>GSDGDYDYLIKFLALGDSGVGKTSVLYQYTDGKFNSKFITTVGIDFREKTIYRNDKRIKLQLWDTAGLERFRSLTTAFFRDAMGFLLLFDLTNEESFLNVRNWISQLKTHAYSENPDIVLCGNKSDLEDERVVAAAEARQLAEHYGIPYFETSAANGTNISQAIEMLLDLIMKRMERSVDKS[16x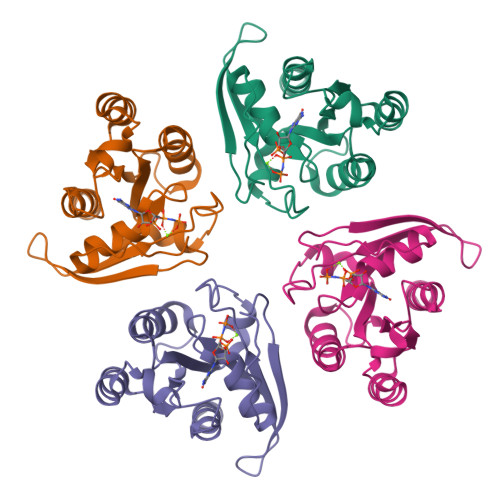]>MEKKVLLTGFDPFGGETVNPSWEAVKRLNGAAEGPASIVSEQVPTVFYKSLAVLREAMKKHQPDIIICVGQAGGRMQITPERVAINLNEARIPDNEGNQPVGEDISQGGPAAYWTGLPIKRIVEEIKKEGIPAAVSYTAGTFVCNHLFYGLMDEISRHHPHIRGGFIHIPYIPEQTLQKSAPSLSLDHITKALKIAAVTA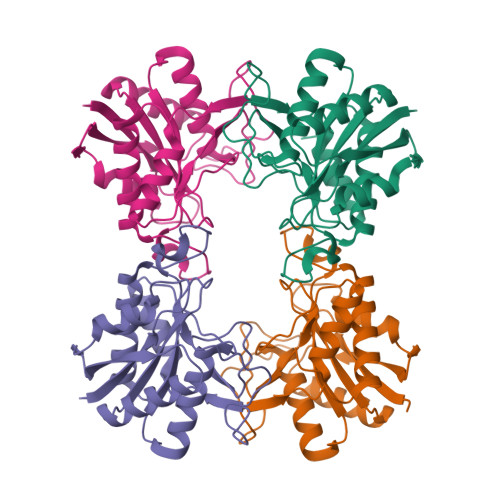AAHEDDIETGGGELHLEHHHHHH[4x]> 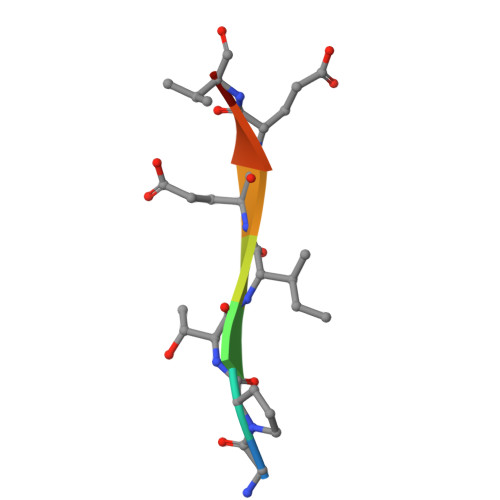GPTIEEVD>SPIIKLRNFNNAIKYILIDKFTRAGDVVLELACGKGGDLRKYGAAGISQFIGIDISNASITEALKRYHSMKNLEYQVILITGDCFGESLGVAVESFPECRFPCDIVSCQFALHYAFETEEKARRMLLNVVKSLKIGGYFFGTIPDSEFIRYKMNKIPESVEKPSWGNSIYKVTFSNNEYQKNGNEFPSPFGQMYTFWLEDAIDNVPEYVIPFESFRSLADEYGMELELQKGFNEFFVEEIPNWVNRFSPKMREGLKRSDGRYGVEGVEKEPAAYFYTTFAFRKVRDYQE[2x]

The essential enzyme messenger RNA (mRNA) (guanine-N7) methyltransferase catalyzes S-adenosylmethionine (SAM)-dependent conversion of GpppRNA ends to the m7GpppRNA cap structure characteristic of eukaryal mRNAs. The antibiotic sinefungin (SFG) is a SAM analog in which the S-CH3 sulfonium moiety of SAM is replaced by a C-NH2 amine. Available evidence indicates that the antifungal activity of SFG is exerted via inhibition of fungal cap methyltransferase Abd1. Crystal structures of K. lactis and S. cerevisiae Abd1 as binary complexes with SAH or SFG and ternary complexes with GTP•SFG highlight how SFG makes two hydrogen bonds from its C-NH2 amine to the guanine-O6 and -N7 atoms of GTP that account for its higher affinity vis-à-vis SAH and SAM.

Here we co-crystallized KlAbd1Δ137 with 0.9 mM m7GTP and determined the structure using KlAbd1Δ137-SAH as a search model. The final model was refined at 1.33 Å resolution with Rwork/Rfree of 18.5/20.3. Electron densities for m7GTP were observed in both methyl acceptor sites. Additional electron densities were observed in the methyl donor sites, which were interpreted as the co-purified adenine moiety of the product SAH. The tertiary structure of m7GTP-bound KlAbd1Δ137 was virtually identical to that of SAH-bound KlAbd1Δ137 (r.m.s.d. of 0.4 Å over 287 Cα positions). The guanine moiety of m7GTP is buried in a deep pocket created by Phe247, Ala248, His250, Phe333, Ile339, and Phe412. The guanine-N1 and -N2 atoms make a bidentate hydrogen bond with the Glu344-Oε1 and Oε2. Guanine-O6 makes direct and water-mediated hydrogen bonds with Tyr251-OH. Guanine-N3 makes a hydrogen bond to Tyr413-OH. The ribose O2′ makes hydrogen bonds with Asn147-Nδ2 and Tyr413-OH.> MNRIISINGPLVIAKGKFSIFEVVRVGEEKLIGEVIGIENDKAYIQVYEDTNGLKVGEPVFNTGKPLTIELGPGLLANIFDGLGRPLKDIYEKTQSIYIPKGIDLPTLDRKKVWEFIPKKKKGDTIKGGDIIGTVNENGFEHRIIVPPNVEGKIEEIYEGNFTIEETIAIVNGKPIKLYHEWPIRKPRPYKEKLDYNYPFITGTRVLDIMFPIAKGGSAAVPGPFGSGKTVLNQQIAKWADSDIVIYIGCGERGNEMTEVLEEFPKLKDPKTGKPLMYRTILIANTSNMPIAAREASI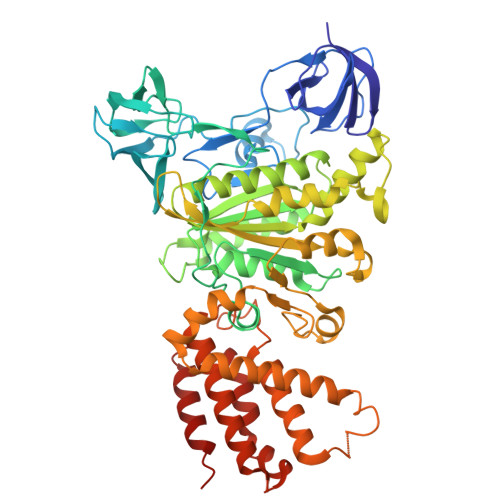YLGATIGEYFRDQGYSVVVNADSTSRWAEALREISSRLGEIPSEEGYPAYLLRKLAEFYERSGRVRTLNDLEGSLTIIGAVSPPGGDFSEPVTQNTLRLVGALWALDSKLAYKRHYPAINYLISYTKQWEFVKKYFEELYEDVIEIREEFFAILKRESELMDIVSIVGPDALSDNEKIYLHMGRIIREGFLQQDAFDENDSYSPLEKTIELMRIIHKYYVTVKQLLGKIPLEEIEQKGIHEKIIKLRYKSLKEFREEIKAIEQEILSLLNSQ> MALFGSNDVTTAHSDYEIVLEGGSSSWGKVKARAKVNAPPASPLLPADCDVKLNVKPLDPAKGFVRISAVFES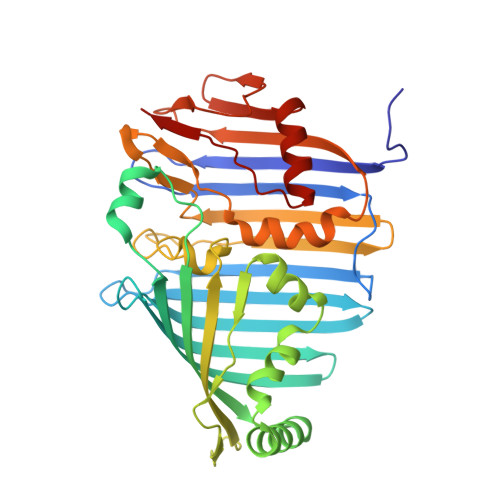IVDSTKNKLTIEADIANETKERRISVGEGMVSVGDFSHTFSFEGSVVNLFYYRSDAVRRNVPNPIYMQGRQFHDILMKVPLDNNDLIDTWEGTVKAIGSTGAFNDWIRDFWFIGPAFTALNEGGQRISRIEVNGLNTESGPKGPVGVSRWRFSHGGSGMVDSISRWAELFPSDKLNRPAQVEAGFRSDSQGIEVKVDGEFPGVSVDAGGGLRRILNHPLIPLVHHGMVGKFNNFNVDAQLKVVLPKGYKIRYAAPQYRSQNLEEYRWSGGAYARWVEHVCKGGVGQFEILYAQ> GPGGSGGVTEEQVHHIVKQALQRYSEDRIGLADYALESGGASVISTRCSETYETKTALLSLFGIPLWYHSQSPRVILQPDVHPGNCWAFQGPQGFAVVRLSARIRPTAVTLEHVPKALSPNSTISSAPKDFAIFGFDEDLQQEGTLLGKFTYDQDGEPIQ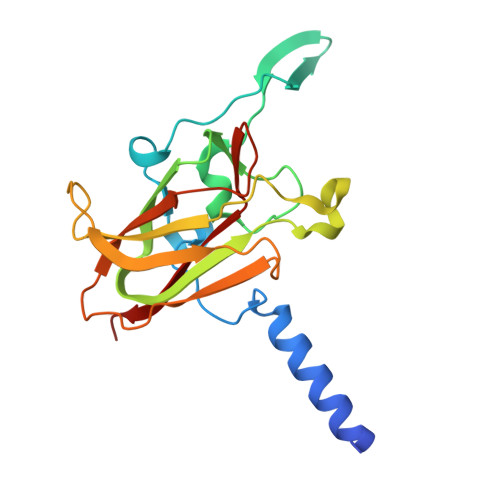TFHFQAPTMATYQVVELRILTNWGHPEYTCIYRFRVHGEPAH> MVSVSPSKVTLPRGGSVLVTCSASCD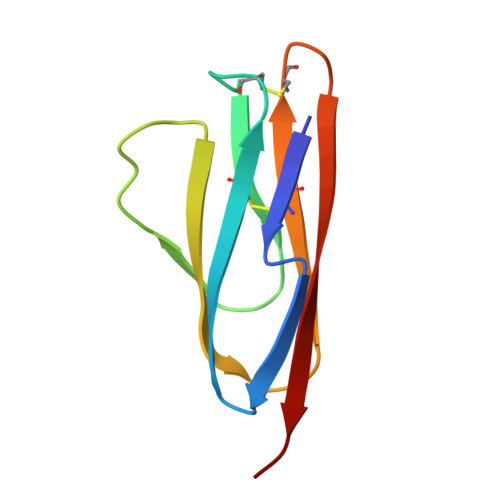QPKLLGIETPLVKKELLLPGNNRKVYELSNVQEDSQVMCYANCPDGQSTAKAFLTVYWT>NNNGA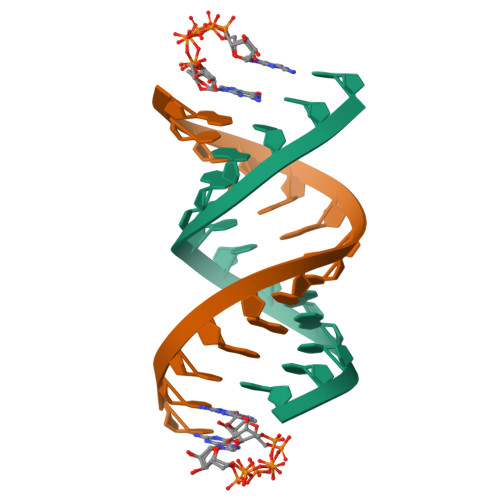CUUAAGUCG[4x]>GQSSNHKENKLPDWAFGGFERPKNVNPVISPIENTKFYCPLTKDSIAWESNDTFNPAATLYNGEIVVLYRAEDKSGVGIGHRTSRLGYATSTDGTHFQREKTPVFYPDNDSQKELEWPGGCEDPRIAVTDDGLYVMMYTQWNRHVPRLAVATSRNLKDWTKHGPAFAKAFDGKFFNLGCKSGSILTEVVKGKQVIKKVNGKYFMYWGEEHVFAATSDDLIHWTPIVNIDGSLKKLFSPRDGYFDSHLTECGPPAIYTPKGIVLLYNGKNHSGRGDKRYTANVYAAGQALFDANDPTRFITRLDEPFFRPMDSFEKSGQYVDGTVFIEGMVYFK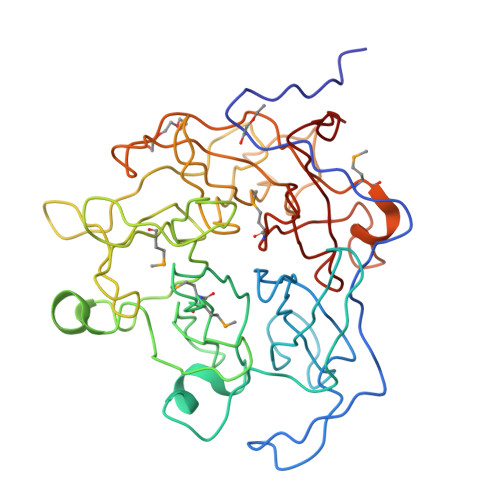NKWYLYYGCADSKVGVAVYDPKRPAKADPLP[2x]>[2x]MNSLLRLPALKRGVFTMSKRGLATTVSPKTRTSNLKNGLTIASESNPLVQTATVGVWIDAGSRNENAYNNGTAHFFEHLAFKGTDKRSQHQLELDIENMGGHLNAYTSRESTVYYAKSFKDDVPKSVEILADILQHSKLAESAIDREREVITRELEEVNKQYEEVVFDHLHATAFMNQPLGRTILGPRENIQTITNTELRKFITENYTADRMVLVGAGAVDHDALVELAEKYFSHLPSSQSPVPLGTPRSSGEDANQNPIPNFVGSEVRLRDDTMPVAHIAIAVEGVSWTSEDYYTALVAQAIIGNYDRAVGTSRHQGSRLSNIVSENNLANSFQSFSTSYSDTGLWGIYLTSENTTQIDDLVHFTLKEWNRLSTSVSNLQVERAKSQLKAGLLLSLDGTTYVAEDIGRQLTTLGRRVTPAEVEAKLEAVTEHDVRAWAQKTLYDKDIALVGLGPIEGLYDYNRIRNDMSMMRW;>MTRGVPRLAVAARHFSTAEAAGVKVAAQDGQSPISDLSVVLRGGSRYATVPGVSHILEKFAFQNTVPKSALRFVRELELFGGKLYTHTTREHIVLRTQFLKQDLPYFVDAFANVLKETKFQQFELTERVAPVAELDLLKRESDPAFTALEAAHEVAFRTGLGNSVYAQGYSPVTLEDVKEFARQVYAKQNVAVVGNNVVPADLQQLVGTAFADLQEGSKVTQAGTTTLHGGEARVRTSTGNALTIALPIAEPKPVYHALASFLGGPASMPWSVGASPLAQATVGTHTSVKATYHNYGDAGLFAITIKGDSPAEISQVAHKAVQALKDTGAEVTEEQAARAYAKSKFAAAEAFENPDSSASVIGMELLSGVSRIAPENVQKFTPAELSEAAAQLSASAKPVVAAVGQVHALPFADELF[2x];>MALRKKNSLLNMANSYVLDSPQPSNLNYFWNFGSLLALCLVIQLATGITLAMHYTSHASLAFDSVEHIMRDVNFGWFIRYAHANTASFFFICIYAHMGRNIYYGSYKTPRVLPWSIGVIIFLLLIITAFMGYVLVFGQMSLWGATVICNLVSAIPWLGEDIVHFLWGGFSVGNPTLQRFFALHYLMPFVLAVFALLHLIALHTAGSSNPLGITSNVDKLSMHPYYSFKDLITVFAFLLMFTLFVFFSPDKLGHPDNYIPANPMVTPASIVPEWYLLPFYAILRAIPDKLGGVIAMVAAILILLILPIVDRSIIRGNAFKPISKLLFGFFICNFLLLGVLGQVHIEPPFIVLGQICTIFYFSYFLILL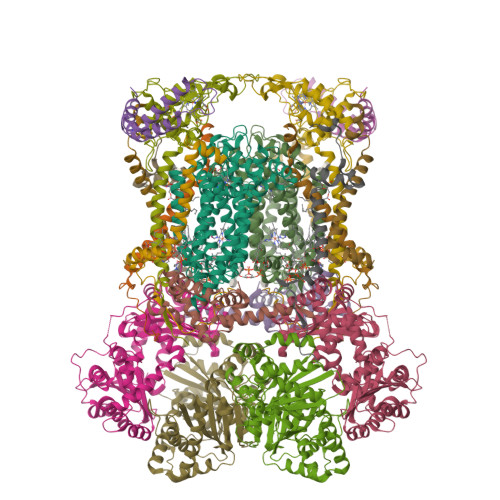PMVSTIENIFFYIGSLRK[2x];>MRRRRIGVWPENRRVSRLWVSLSPRSCVTCPVPTNQNPPINNHHTPILTQMFKAIPLRQALLGISSAVCAGATTTYYYTTKAEAMTAAEHGLHPAEYPWPQNGMLSTFDHASLRRGYQVYKEVCAACHSLDRIAWRNLVGVTHTTDEAKAFAEELEYDDEPDDEGNPRKRPGKLADYIPGPYPNEQAARAANQGALPPDLSLIAKARHGGADYIFALLTGYPDEPPAGVVLAPGMNYNPYFPGGGIGMARTLFDGVVEYEDGTPATTSQMAKDVAAFLTWAAEPEHDERKKLGLKAIIVISAMLGLSVYIKKFKWSPIKNRKFIYNPPKN[2x];>[2x]MSLLRTAAQAVKAPKAYTPLVAAKAFAQTRSVSSQPIGGKSTYKIPDFTPYLKKDRNTDANRLFSYFMIGSFGMLSAAGAKATVQDFLSNMSASADVLAMAKVEVKLGAIPLGKNVIIKWRGKPIFIRHRTSEEIEEANEVNVATLRDPQTDDERVQKPEWLVMIGVCTHLGCVPIGEAGDFGGWFCPCHGSHYDISGRIRRGPAPLNLEIPEYDFADAETLVIG;>[2x]MSYFLTLASEVAESLLPTVAFASEEEKEQDEPVEVESDDDESEEKEDDDEEEDEDDDDDDDDDEVPDPAIALHEAAAEGPCHDFKHHFDECVERVTKAQEAEDYDHAEYKEDCVEEFFHLQHCINDNTADKLFRVLK;>[2x]MASITSVVKTSELILKSPLLSKIVVPLAKTYVKFSGYRQLGFKMNDLIIEETPNMQLALRRLPPTESYDRVYRLIRATQFSLSHKLATGNDITKPEEDDHYLIPYILDVEAEAFEKDALDNLEVVKRK;>MGGNGHYMGWWGHMGSPPQKGIAGYTISPFAARPFAGVVHAAIFNTFRRTKNQALFVILPVSFFYYVWTQASEKNEWLYTKAGRHELAKALAE[2x];>[2x]MAWATTFYNVFVKRNSAFVATILASAFVFDMTFETAIDNFWDRINAGKQWKDIRHKYIEAAGDDDEDDE;>[2x]MICGEGDYVKKPSYKIVPHFLGFNIPTVSKWIPIFGIWGAAAGIGALFLIEGVPRTRQDILSKIPIIGEHWIREIPASDNPF> MRGSHHHHHHENLYFQGSLAVAEPVVNAADAKGTNVNDKVTASDFKLEKTAFDPNQSGNTFMAANFKVTGQVKSGDYFTAKLPDSVTGNGDVDYSNSNNTMPIADIKSTNGDVVAKATYDILTKTYTFVFTDYVNDKENINGQFSLPLFT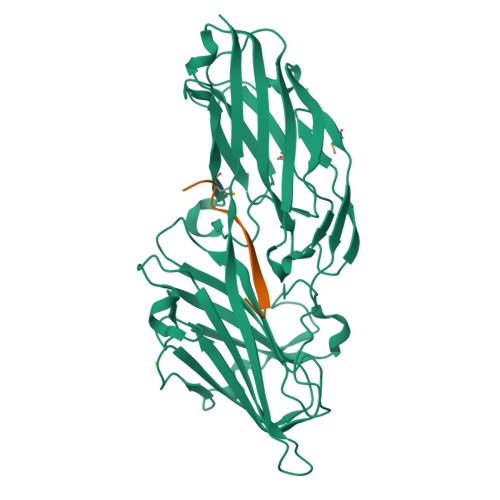DRAKAPKSGTYDANINIADEMFDNKITYNYSSPIAGIDKPNGANISSQIIGVDTASGQNTYKQTVFVNPKQRVLGNTWVYIKGYQDKIEESSGKVSATDTKLRIFEVNDTSKLSDSYYADPNDSNLKEVTGEFKDKISYKYDNVASINFGDINKTYVVLVEGHYDNTGKNLKTQVIQENIDPATGKDYSIFGWNNENVVRYGGGSADGDSAVN;> ASGSSGTGSTGNQ>GPLGSPSENIQEINTAISDNYTYNIPGIVNNNPFYILFTVNTTGIYKINAQNNLPSLKIYEAIGSGNRNFQSGNLCDDDIKAINYITGFDSPNAKSYLVVLLNKDKNYYIRVPQTSSNIENQIQFKREEGDLRNLMNSSVNIIDNLNSTGAHYYTRQSPDVHDYISYEFTIPGNFNNKDTSNIRLYTSYNQGIGTLFRVTETIDGYNLINIQQNLHLLNNTNSIRLLNGAIYILKVEVTELNNYNIRLHIDITN[4x];>[4x]GPSVERTFLPNGNYNIKSIFSGSLYLNPVSKSLTFSNESSANNQKWNVEYMAENRCFKISNVAEPNKYLSYDNFGFISLDSLSNRCYWFPIKIAVNTYIMLSLNKVNELDYAWDIYDTNENILSQPLLLLPNFDIYNSNQMFKLEKI

Here, we report the complete structure of a bimodular ∼760 kDa BoNT/A large progenitor toxin complex (L-PTC), which is composed of BoNT and four non-toxic bacterial proteins. We found that L-PTC/A consists of two structurally and functionally independent sub-complexes, the M-PTC and the HA complex. The HA complex is composed of HA70, HA17, and HA33 in a 3∶3∶6 stoichiometry and adopts an extended three-blade architecture, whereas the M-PTC is situated on top of the HA complex platform. BoNT/A absorption is mainly mediated by nine glycan-binding sites on the HA complex that together form multivalent interactions with host carbohydrate receptors on intestinal epithelial cells.

We also obtained a high-resolution structure of the blade by combining the structures of HA70D3–HA17 and HA17–HA33, which were determined at 2.4 Å and 2.1 Å, respectively. Based on the crystal structure of the HA70D3–HA17 complex, the interactions between HA70 and HA17 bury a solvent-accessible area of ∼795 Å2 (per molecule). The structure of HA70D3 is almost identical to its equivalent domain in the full-length HA70 with a root-mean-square deviation (rmsd) of ∼0.93 Å over 232 Cα atoms. The major HA70–HA17 interactions are composed of 13 pairs of hydrogen bonds and salt bridges. In addition, HA70-Phe547 is buried in a hydrophobic region in HA17 composed of Ile18, Ile92, Ala93, Thr96, and Met140. HA17 has a compact β-trefoil fold and connects HA70 and HA33.> MGAMIVKEVYETAEKIKSMEIRGAGRIARAAAQALMIQAEKSKAKEPEELWNELKVASKILYNTRPTAVSLPNALRYVMHRVKAAYLGGADLETLRFTAINSAKEFIYNSEKAIERIGEIGAKRIEDGDIIMTHCHSKAAISVMKKAFEQGKNIKVIVTETRPKWQGKITAKELASYGIPVIYIVDSAARHYMKMTDKVVMGANSITANGAVINKIGTSLIALTAKEHRVWVMIAAETYKFHPATMLGQLVEIEMRDPTEVIPEEELRTWPKNIEVWNPAFDVTPPEYIDVIITERGIIPPYAAIDILKEEFGWALKYKEPWED

In summary, our study demonstrates that PH0208 protein would function as a purine nucleotide dependent R15Pi enzyme and not as a homologue of the regulatory subunit of eIF2B. In NMP degradation pathway, R15Pi catalyzes the conversion of ribose-1,5-bisphosphate (R15P, substrate) into ribulose-1,5-bisphosphate (RuBP, product) in an adenosine 5′-monophosphate (AMP)-dependent manner. AMP acts as an activator of R15Pi and in its absence the enzymatic activity has been found to decline dramatically. Monomer of PH0208 protein consists of an N-terminal α-helical domain (residues 1–122) and a C-terminal α-β-α sandwich domain (residues 123–324).

To identify the binding site of ribonucleotides, either co-crystallization or soaking of PH0208-WT, PH0208-C135S and PH0208-D204N proteins with AMP, GMP, CMP and TMP was performed. Complex of AMP and GMP bound to the proteins were obtained, however, no electron density for CMP or TMP was observed. Mutation of the two catalytic residues (Cys135 and Asp204) did not alter the binding behavior of AMP to the protein. In case of both the mutants, PH0208-C135S and PH0208-D204N, AMP occupies a similar position to that of PH0208-WT protein with the major interactions arising from the three subunits of the hexamer. Similar to PH0208-WT, the adenosine base ring interacts with Val251 of chain B, the oxygen atoms of ribose sugar interacts with Arg124 & Asp290 of chain A and Asn209 of chain B while the phosphate group forms hydrogen bond with Arg229 & Trp231 of chain A and Arg190 & Lys194 of chain D of the mutant proteins. Thus, it might also be possible that the binding of GMP to the ‘GMP binding loop’ is an outcome of crystallization artifact. Both, AMP and GMP bind to PH0208 protein even after the mutation of the catalytic residues (PH0208-C135S and PH0208-D204N) at the active site pocket.>GFEKYWFCYGIKCYYFDMDRKTWSGCKQTCQISSLSLLKIDNEDELKFLQNLAPSDISW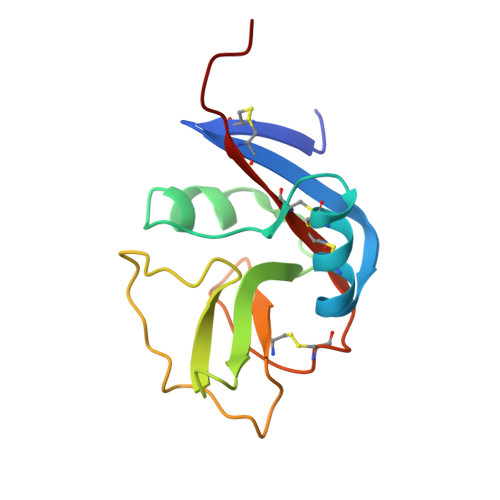IGFSYDNKKKDWAWIDNGPSKLALNTTKYNIRDGLCMSLSKTRLDNGDCGKSYICICGKRLDKFPH[2x]>MVSTDWKSDLRQRGYRLTPQRQLVLEAVDTLEHATPDDILGEVRKTASGINISTVYRTLELLEELGLVSHAHLGHGAPTYHLADRHHHIHLVC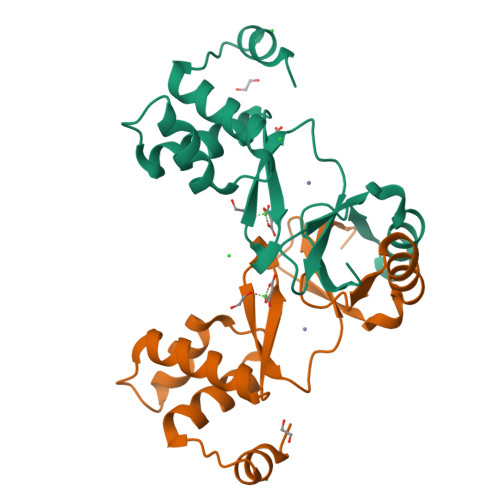RDCTNVIEADLSVAADFTAKLREQFGFDTDMKHFAIFGRCESCSLKGSTTDS[2x]> MGIINIQDEINNYMKEVYGATTVKSTYDPSFKVFNESVTPQFTEIPTEPVNNQLTTKRVDNTGSYPVESTVSFTWTETHTE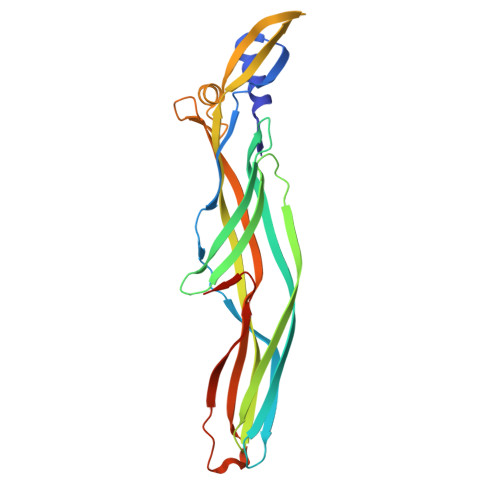TSAVTEGVKAGTSISTKQSFKFGFVNSDVTLTVSAEYNYSTTNTTTTTETHTWSDSTKVTIPPKTYVEAAYIIQNGTYNVPVNVECDMSGTLFCRGYRDGALIAAVYVSVADLADYNPNLNLTNKGDGIAHFKGSGFIEGAQGLRSIIQVTEYPLDDNKGRSTPITYLINGSLAPNVTLKNSNIKF(2R,3R,4S,5S)-2-(6-amino-9H-purin-9-yl)-5-[(benzyldisulfanyl)methyl]tetrahydrofuran-3,4-diol 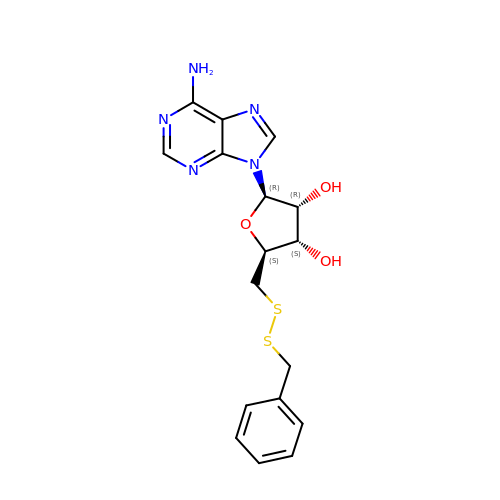| C17 H19 N5 O3 S2 | DBQUNXDCOIKHGM-LSCFUAHRSA-N8-METHOXY-1-METHYL-4-(4-(4-(1-METHYLPYRIDINIUM-4-YLAMINO)PHENYLCARBAMOYL)PHENYLAMINO)QUINOLINIUM | C30 H47 N5 O2 | 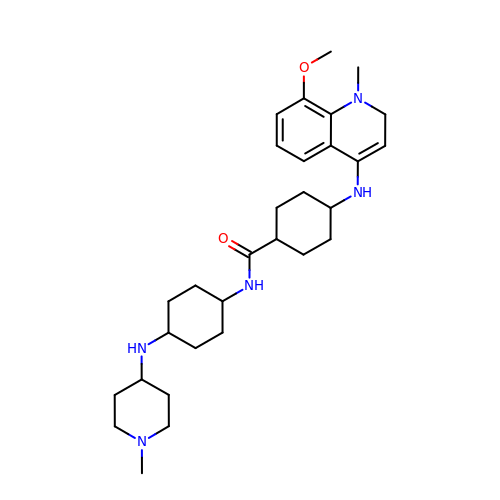LXOIZJXCTNTVJO-XQINFXQGSA-N> GGSADPLRERTELLLADYLGYSAREPGTPEPAPSTPEAAVLRSAAARLRQIHRSFFSAYLGYPGNRFELVALMADSVLSDSPGPTWGRVVTLVTFAGTLLERGPLVTARWKKWGFQPRLKEQEGDVA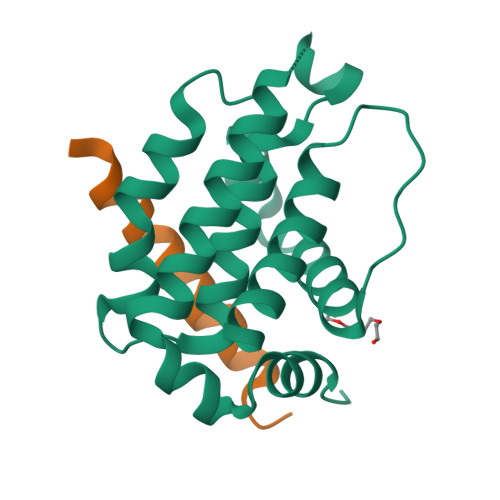RDSQRLVALLSSRLMGQHRAWLQAQGGWDGFSHFFRTPFPLAENLYFQ;> GSDMRPEIWIAQELRRIGDEFNAYYARR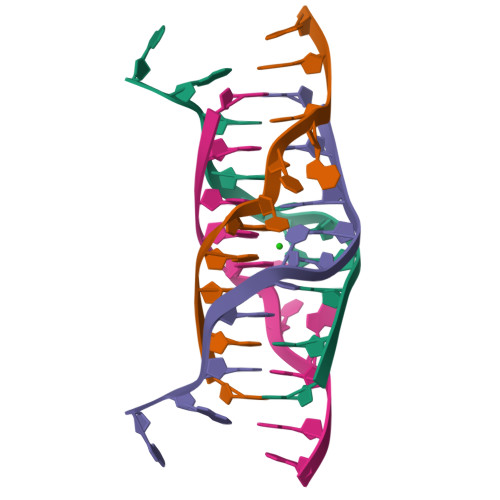>[2x]CCAGGCTGCAA Of these, the MT-based motor, Kinesin-5 plays a key role, being essential for the assembly of bipolar spindles in most eukaryotic cells and driving or constraining the rate of spindle elongation. Purified, native Kinesin-5 is a ‘slow’, plus-end-directed, bipolar, homotetrameric motor capable of using pairs of N-terminal motor domains at opposite ends of a central rod to crosslink MTs into bundles. Structure-function analysis of the Drosophila melanogaster Kinesin-5, KLP61F, identified a central bipolar assembly (BASS) domain within the coiled-coil rod that is critical for this motor’s bipolar organization and whose deletion results in disassembled, mostly monomeric, Kinesin-5. Instead of the expected antiparallel arrangement of two side-by-side parallel coiled-coils proposed previously, we find that the BASS domain has a novel four-helix bundle structure, which very likely has important implications for its mechanism of action within the spindle.

We purified a minimal BASS domain construct that assembles into a tetrameric, 220 Å long rod based on EM (KLP61F residues 635–835). This BASS tetramer formed hexagonal (P6422) crystals, which were used to determine its structure to 2.6-Å resolution using X-ray crystallography with the single wavelength anomalous dispersion (SAD) method from selenomethionine-and mercury-derived crystals. The asymmetric unit contains a canonical anti-parallel coiled-coil BASS domain dimer encompassing residues 640–802 of both chains, which represents the basic assembly unit of a Kinesin-5 minifilament. This anti-parallel dimer is associated with a second dimer through a crystallographic dyad axis to form the full tetramer, whose dimer–dimer packing surface extends over a large area (≈7000 Å2) and is stabilized by sequential, alternating hydrophobic and ionic residue interfaces, each occupying three-helical turns. The resulting four-helix bundle, which is 22 Å wide, 26 Å high, and 260 Å long is the longest helical minifilment structure determined to date, and it displays a striking organization. It consists of a 220-Å-long central bundle that is visible by EM and matches fairly well to other anti-parallel four-helix bundles, where helical axes are separated by equal distances but then transitions to an asymmetric diamond-shaped bundle near its ends, where C-terminal helical axes become displaced and N-terminal helical axes are closer mediated by helical bends, termed elbows. The hydrophobic central interface (A) is bracketed by an ionic interface (B), another hydrophobic interface (C), and finally another ionic interface (D) positioned at the ‘elbows’ marking the transition between anti-parallel four-helix bundle and parallel coiled-coils at the ends.

>[2x]MQQQQLLMSKEIQTNLQVIEENNQRHKAMLDSMQEKFATIIDSSLQSVEEHAKQMHKKLEQLGAMSLPDAEELQNLQEELANERALAQQEDALLESMMMQMEQIKNLRSKNSISMSVHLNKMEESRLTRNHRIDDIKSGIQDYQKLGIEASQSAQAELTSQMEAGMLCLDQGVANCSMLQVHMKNLNQKYEKETNENVGSVRVSGHHHHHH> MSASAQQLAEELQIFGLDCEEALIEKLVELCVQYGQNEEGMVGELIAFCTSTHKVG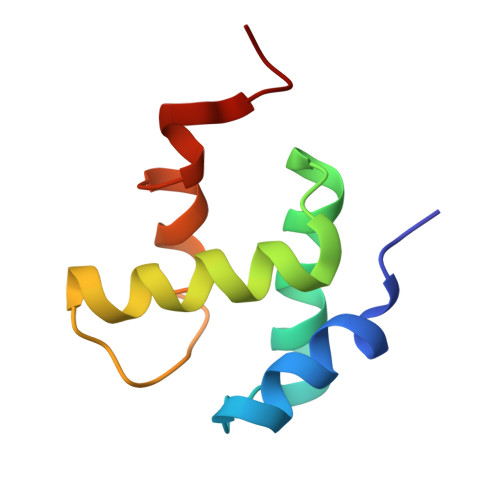LTSEILNSFEHEFLSKRLSKAR> QAKHKQRKRLKSSCKRHPLYVDFSDVGWNDWIVAPPGYHAFYCHGECPFPLADHLNSTNHAIVQTLVNSVNSKIPKACCVPTELSAISMLYLDENEKVVKKDYQDMVVEGCGCR;> QNLDSMLHGTGMKSDSDQKKSENGVTLAPEDTLPFLKCYCSGHCPD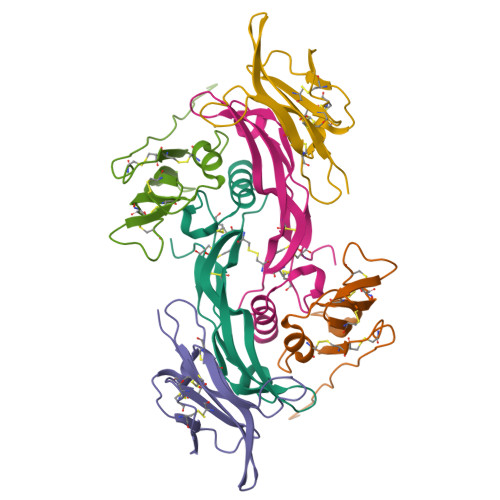DAINNTCITNGHCFAIIEEDDQGETTLASGCMKYEGSDFQCKDSPKAQLRRTIECCRTNLCNQYLQPTLPPVVIGPFFDGSIR;> SGRGEAETRECIYYNANWELERTNQSGLERCEGEQDKRLHCYASWRNSSGTIELVKKGCWLDDFNCYDRQECVATEENPQVYFCCCEGNFCNERFTHLP>[4x]MDFSKMSIVGRIGSEFTEHTSANNNRYLKYSIASQPRRDGQ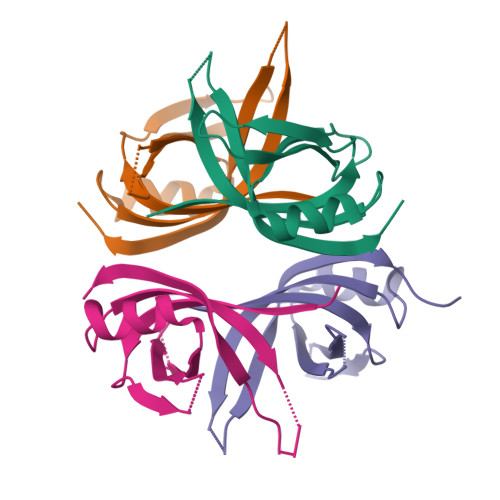TNWYNITVFNEPQINFLTEYVRKGALVYVEADAANYVFERDDGSKGTTLSLVQKDINLLKNGKKLEDAEGQENAASSE>MSNAEKALGVALIGTGFMGKCHAMAWRNVATAFGGLPPRLEVLADMPADKAHSLASSFGFARGTADWREAVSDPAVDVVSITTPNGLHREMAEAALAAGKHVWLEKPMALSVEDAQAMEAAARASDRRTIIGYNYTRSPAFRAAVDLIAEGAIGRPIHFRGMYDEDYMADPDLPWSWRLTRKDGGLGALGDLGCHLVSVMVSLMGPVARVYAQADTVITDRPHQGGTARVENEDQAQALIRFASGTSGEFSCSRVARGYRCRLAWEVQGTEGTLRFDQERMNELWLYQ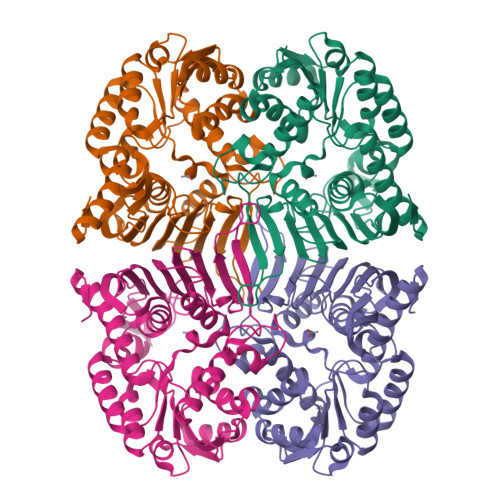PGRPEIDGFRRILTGPAQPGFAAFCPGGGHNFGFNEQKVVEAEMLRQAIAGRGKAWPDFTDGLTIERVIHGMATSAQTGQPVNFLEHHHHHH[4x]> LNPKIIIFEQENFQGHSHELNGPCPNLKETGVEKAGSVLVQAGPWVGYEQANCKGEQFVFEKGEYP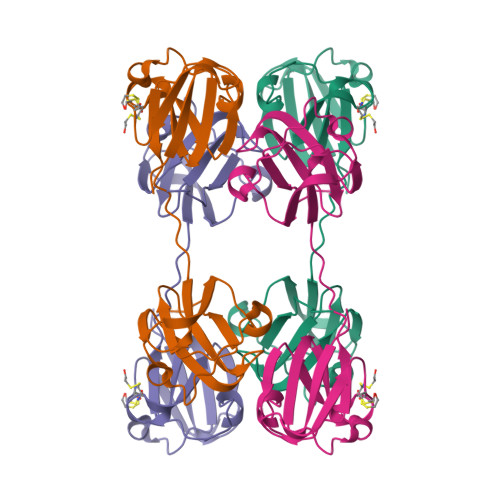RWDSWTSSRRTDSLSSLRPIKVDSQEHKITLYENPNFTGKKMEVIDDDVPSFHAHGYQEKVSSVRVQSGTWVGYQYPGYRGLQYLLEKGDYKDSGDFGAPQPQVQSVRRIRDMQW>MSENTYPSVNDLTLEEKASLTSGGDAWHLQGVEAKGIPGYMITDGPHGLRKSNSATTGEVDLNNSVPATCFPPAAGLSSSWNPELIHQVGEAMAEECIQEKVAVILGPGVNIKRNPLGGRCFEYWSEDPYLAGHEAVGIVAGVQSKGVGTSLKHFAANNQETDRLRVSANISQRALREIYFPAFEHIVKTAQPWTIMCSYNRINGVHSAQNRWLLTDVLRDEWGYEGIVMSDWGADHDRVASLNAGLNLEMPPSYTDDQIVYAARDGRIQPEQLDRMAQGMVDLVNKTRSAMSIDDYHFDVDAHDEVAHQAAIESMVLLKNDDDILPVAANAKIAVIGEFARTPRYQGGGSSHITPTKMTSFLDTLAARGVDVAFAPGFTLDLEPADRTLEAEAVETAKNADVVLMFLGLPEAAESEGFDRETLDIPAKQVELL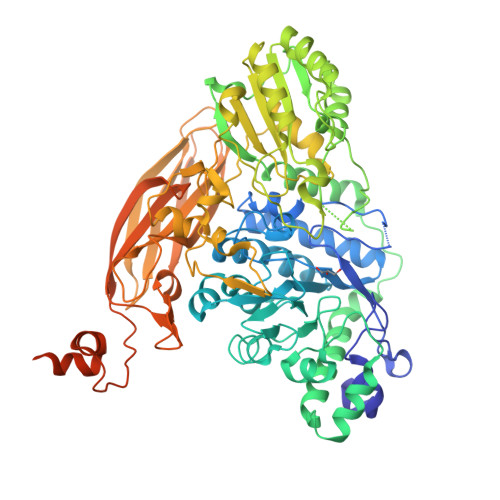KAVAAENKNIVVVLSNGSVVSVAPWAGNAKGILESWLLGQAGGPALADVIFGKVSPSGKLAQTIPMNINDDPSMINWPGEEGHVDYGEGVFVGYRYYDTYDKAVDYPFGFGLSYATFAIDGVNVAKTGANTAHVTATVTNTSDVDAAETVQVYVAPGKAAVARPKHELKGFRKVFLKAGESAEITFDLDERAFAYWSEKFNDWHVEAGEYTVEVGTSSRDIAAVAVVTLDGDGKALPLDEWSTFGEWADDPVGSKIVASVYAEGEAGNLPQLPDNDMMRMFLKSMPINSMPMLMSDGGKAITAFMLDEYAKIAETAE[4x]> GEEDLCAAFNVICDNVGKDWRRLARQLKVSDTKIDSIEDRYPRNLTERVRESLRIWKNTEKENATVAHLVGALRSCQMNLVADLVQEVQQ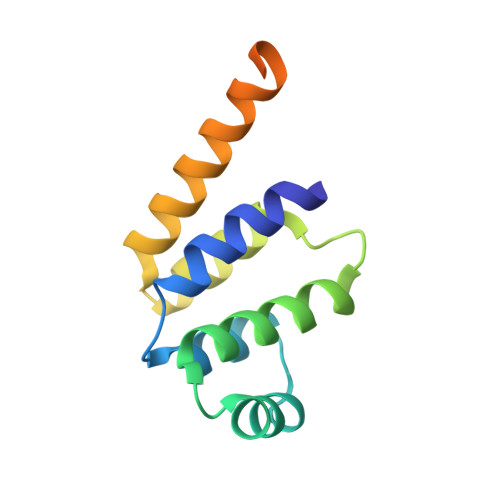ARDLQNRSGAMSPMSWNSDASTSEASHHHHHH>[7x]MAIAQLATEYVFSDFLLKEPTEPKFKGLRLELAVDKMVTCIAVGLPLLLISLAF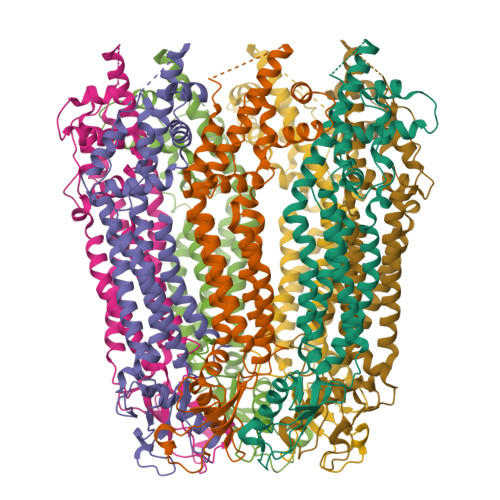AQEISIGTQISCFSPSSFSWRQAAFVDSYCWAAVQQKNSLQSESGNLPLWLHKFFPYILLLFAILLYLPPLFWRFAAAPHICSDLKFIMEELDKVYNRAIKAAKSARDLDMRDGACSVPGVTENLGQSLWEVSESHFKYPIVEQYLKTKKNSNNLIIKYISCRLLTLIIILLACIYLGYYFSLSSLSDEFVCSIKSGILRNDSTVPDQFQCKLIAVGIFQLLSVINLVVYVLLAPVVVYTLFVPFRQKTDVLKVYEILPTFDVLHFKSEGYNDLSLYNLFLEENISEVKSYKCLKVLENIKSSGQGIDPMLLLTNL During the site-specific DNA recombination reaction that excises phage λ from the chromosome, the bacterial DNA architectural protein Fis recruits multiple λ-encoded Xis proteins to the attR recombination site. Fis is a bacterial nucleoid protein that functions in transcription, replication, and recombination reactions. Xis is a winged-helix DNA binding protein, which is expressed at high levels shortly after prophage induction, but by itself, exhibits low binding specificity. To explore the structural basis for Fis recruitment of Xis to the X2 site within the λ prophage attR recombination site, X-ray crystal structures of three different Fis–Xis–DNA complexes were determined.

The ‘FX2’ structure contains a Fis dimer, an Xis1–55 monomer (hereafter referred to as Xis), and a 27 bp DNA duplex representing the native sequence except for an A/T base pair at each end. The most important base-specific contact by Fis in high affinity Fis binding sites is mediated by the guanidinium group of Arg85 to a guanine, and in the FX2 structure, both the N7 and O6 atoms of G7b are within 3 Å. Thus, each base of the position 7 C/G pair is directly contacted by either Fis or Xis (Glu19-C7:N4, 2.7 Å). The Arg23 side chain is present in both conformations in the FX2 complex with the dominant rotamer contacting the DNA backbone, as is the case for the X2 site within the X2–X1.5–X1 microfilament structure. The FX2 structure reveals for the first time a layer of interconnected solvent molecules spanning most of the major groove interface with Fis. Our three crystal structures of Fis and Xis bound to the F-X2 DNA segment reveal little (70 Å2 in the FX2 structure) or no (both FX1-2 structures) shared surface between the Xis and Fis proteins. The closest approach in the FX2 structure is between the polar end of the Xis Gln6 side chain from helix A and the Fis Leu79 side chain methyl, which emanates from its positioning helix C. The 27 bp DNA in the FX2 structure exhibits an overall curvature of 61° (calculated by CURVES), which is within the lower range of bending angles measured in X-ray structures of Fis bound to different DNA sequences. The DNA backbone over the outer 4 bp of FX2 that is proximal to the Xis basic surface (Xis residues Arg14, Arg16, Arg23, Arg29 and Lys49) is then pulled up to 6 Å closer to Xis relative to the Fis-F1 complex, enabling hydrogen bonding by Xis Ser17, Thr20 and Trp24 to proximal phosphates. The result is a snug fit between the peptide backbone and the minor groove surface (surface complementarity score between the Xis wing motif and DNA in the FX2 structure is 0.826).

>[2x]MFEQRVNSDVLTVSTVNSQDQVTQKPLRDSVKQALKNYFAQLNGQDVNDLYELVLAEVEQPLLDMVMQYTRGNQTRAALMMGINRGTLRKKLKKYGMN;> MYLTLQEWNARQRRPRSLETVRRWVRESRIFPPPVKDGREYLFHESAVKVDLNRP> HHHHHHMPFTLGQRWISDTESELGLGTVVAVDARTVTLLFPSTGENRLYARSDSPVTRVMFNPGDTITSHDGWQMQVEEVKEENGLLTYIGTRLDTEESGVALREVFLDSKLVFSKPQDRLFAGQIDRMDRFALRYRARKYSSEQFRMPYSGLRGQRTSLIPHQLNIAHDVGRRHAPRVLLADEVGLGKTIEAGMILHQQLLSGAAERVLIIVPETLQHQWLVEMLRRFNLRFALFDDERYAEAQHDAYNPFDTEQLVICSLDFARRSKQRLEHLCEAEWDLLVVDEAHHLVWSEDAPSREYQAIEQLAEHVPGVLLLTATPEQLGMESHFARLRLLDPNRFHDFAQFVEEQKNYRPVADAVAMLLAGNKLSNDELNMLGEMIGEQDIEPLLQAANSDSEDAQSARQELVSMLMDRHGTSRVLFRNTRNGVKGFPKRELHTIKLPLPTQYQTAIKVSGIMGARKSAEDRARDMLYPERIYQEFEGDNATWWNFDPRVEWLMGYLTSHRSQKVLVICAKAATALQLEQVLREREGIRAAVFHEGMSIIERDRAAAWFAEEDTGAQVLLCSEIGSEGRNFQFASHMVMFDLPFNPDLLEQRIGRLD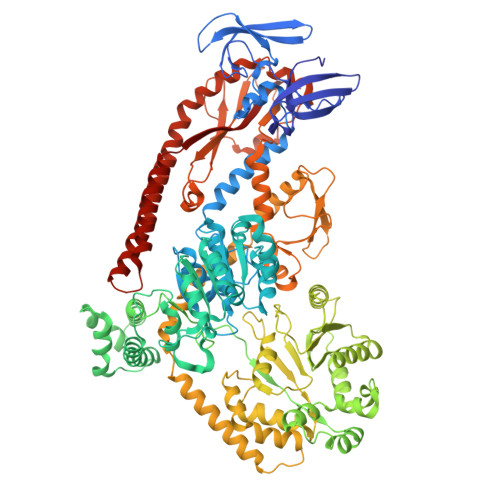RIGQAHDIQIHVPYLEKTAQSVLVRWYHEGLDAFEHTCPTGRTIYDSVYNDLINYLASPDQTEGFDDLIKNCREQHEALKAQLEQGRDRLLEIHSNGGEKAQALAESIEEQDDDTNLIAFAMNLFDIIGINQDDRGDNMIVLTPSDHMLVPDFPGLSEDGITITFDREVALAREDAQFITWEHPLIRNGLDLILSGDTGSSTISLLKNKALPVGTLLVELIYVVEAQAPKQLQLNRFLPPTPVRMLLDKNGNNLAAQVEFETFNRQLNAVNRHTGSKLVNAVQQDVHAILQLGEAQIEKSARALIDAARNEADEKLSAELSRLEALRAVNPNIRDDELTAIESNRQQVMESLDQAGWRLDALRLIVVTHQ> MKEFYLTVEQIGDSIFERYIDSNGRERTREVEYKPSLFAHCPESQATKYFDIYGKPCTRKLFANMRDASQWIKRMEDIGLEALGMDDFKLAYLSDTYNYEIKYDHTKIRVANFDIEVTSPDGFPEPSQAKHPIDAITHYDSIDDRFYVFDLLNSPYGNVEEWSIEIAAKLQEQGGDEVPSEIIDKIIYMPFDNEKELLMEYLNFWQQKTPVILTGWNVESFAIPYVYNRIKNIFGESTAKRLSPHRKTRVKVIENMYGSREIITLFGISVLDYIDLYKKFSFTNQPSYSLDYISEFELNVGKLKYDGPISKLRESNHQRYISYNIIAVYRVLQIDAKRQFINLSLDMGYYAKIQIQSVFSPIKTWDAIIFNSLKEQNKVIPQGRSHPVQP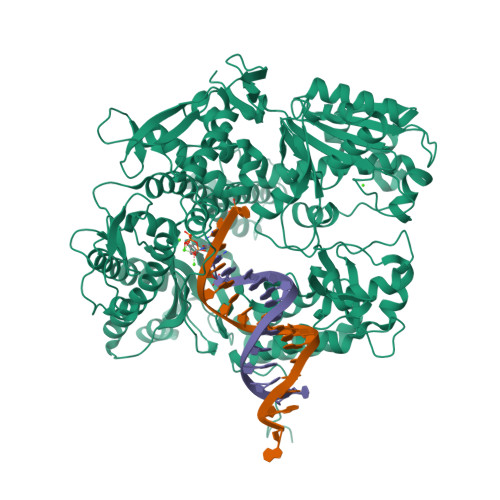YPGAFVKEPIPNRYKYVMSFDLTSLYPSIIRQVNISPETIAGTFKVAPLHDYINAVAERPSDVYSCSPNGMMYYKDRDGVVPTEITKVFNQRKEHKGYMLAAQRNGEIIKEALHNPNLSVDEPLDVDYRFDFSDEIKEKIKKLSAKSLNEMLFRAQRTEVAGMTAQINRKLLINSLAGALGNVWFRYYDLRNATAITTFGQMALQWIERKVNEYLNEVCGTEGEAFVLYGDTDSIYVSADKIIDKVGESKFRDTNHWVDFLDKFARERMEPAIDRGFREMCEYMNNKQHLMFMDREAIAGPPLGSKGIGGFWTGKKRYALNVWDMEGTRYAEPKLKIMGLETQKSSTPKAVQKALKECIRRMLQEGEESLQEYFKEFEKEFRQLNYISIASVSSANNIAKYDVGGFPGPKCPFHIRGILTYNRAIKGNIDAPQVVEGEKVYVLPLREGNPFGDKCIAWPSGTEITDLIKDDVLHWMDYTVLLEKTFIKPLEGFTSAAKLDYEKKASLFDM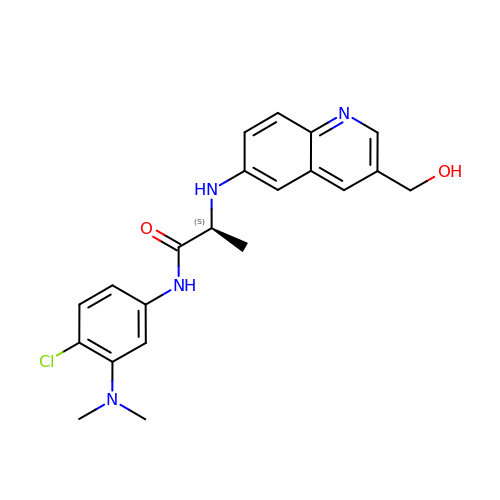N-[4-chloro-3-(dimethylamino)phenyl]-N~2~-[3-(hydroxymethyl)quinolin-6-yl]-L-alaninamide | C21 H23 Cl N4 O2 | DPOWTSNHUDZSRA-ZDUSSCGKSA-N> MISSIRLDLFRTKVFVMPLKFPLSICLLGTFLVTSAQAQEAVKGVVELFTSQGCASCPPAD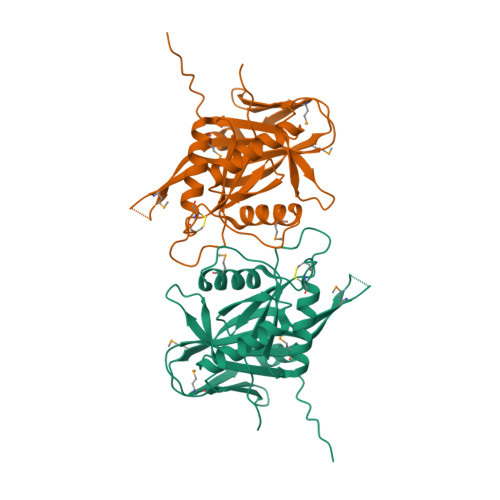EALRKMIQKGDVVGLSYHVDYWNYLGWTDSLASKENTERQYGYMRALGRNGVYTPQAILNGRDHVKGADVRGIYDRLDAFKREGQGLNVPVSSKFAGDEVEIDIGAGNGKADVVVAYFTREQTVDVQKGENQGKKMSYWHSVYDVQTVGMWDGSPMTVKLPASVVAKVKKGGCAVLLQTANASGDPAAIVGASILLGNETQLEHHHHHH> MVRGIRGAITVEEDTPEAIHQATRELLLKMLEANGIQSYEELAAVIFTVTEDLTFAFPAEAARQIGMHRVPLLSAREVPVPGSLPRVIRVL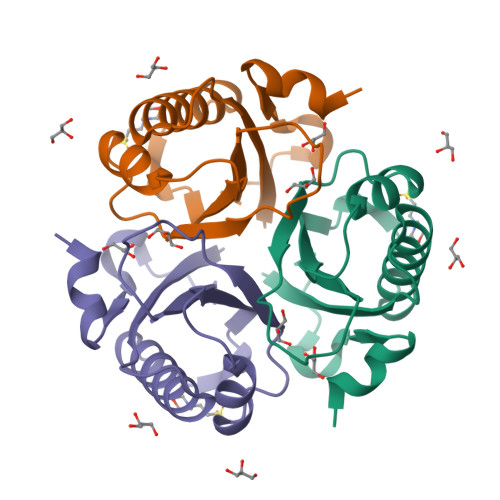ALWNTDTPQDRVRHVYLREAVRLRPDLESAQ>[4x]MSSASGLRRGHPAGGEENMTETDAFYKREMFDPAEKYKMDH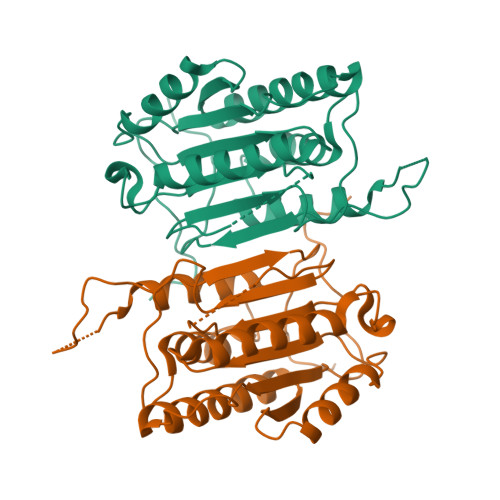RRRGIALIFNHERFFWHLTLPERRGTCADRDNLTRRFSDLGFEVKCFNDLKAEELLLKIHEVSTVSHADADCFVCVFLSHGEGNHIYAYDAKIEIQTLTGLFKGDKCHSLVGKPKIFIIQACRGNQHDVPVIPLDVVDNQTEKLDTNITEVDAASVYTLPAGADFLMCYSVAEGYYSHRETVNGSWYIQDLCEMLGKYGSSLEFTELLTLVNRKVSQRRVDFCKDPSAIGKKQVPCFASMLTKKLHFFPKSN> SMGRAWDGLWDPTLPMIPSANIPGDPIAVVNQVLGISATSAQVTANMGRKFLEQLGILQPTDTGITNAPAGSAQGRIPRVYGRQASEYVIRRGMSQIGVPYSWGGGNAAGPSKGIDSGAGTVGFDASG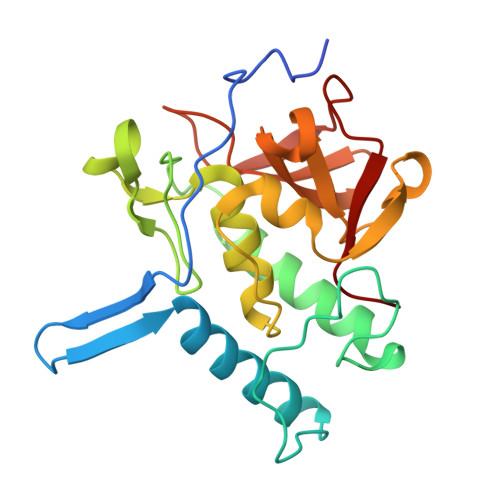LVLYSFAGVGIKLPHYSGSQYNLGRKIPSSQMRRGDVIFYGPNGSQHVTIYLGNGQMLEAPDVGLKVRVAPVRTAGMTPYVVRYIEY> SEKLTFKTDLEKLEREKAAQIGVAIVDPQGEIVAGHRMAQRFAMCSTFKFPLAALVFERIDSGTERGDRKLSYGPDMIVEWSPATERFLASGHMTVLEAAQAAVQLSDNGATNLLLREIGGPAAMTQYFRKIGDSVSRLDRKEPEMNDNTPGDLRDTTTPIAMARTV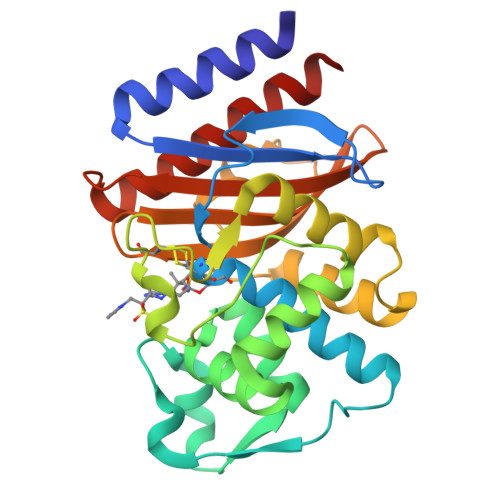AKVLYGGALTSTSTHTIERWLIGNQTGDATLRAGFPKDWVVGEKTGTCANGGRNDIGFFKAQERDYAVAVYTTAPKLSAVERDELVASVGQVITQLILSTDK>[5x]GVSKTFKDKCAS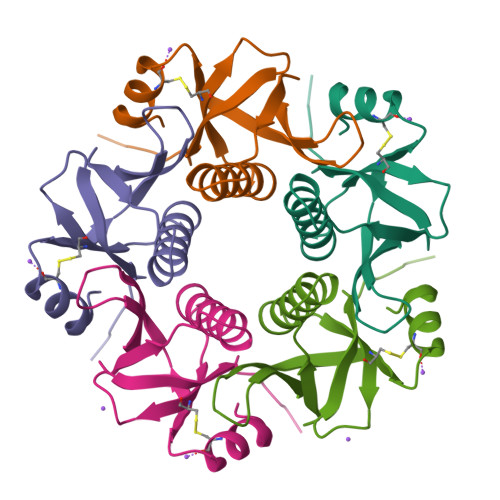TTAKLVQSVQLVNISSDVNKDSKGIYISSSAGKTWFIPGGQYYPDNYLSNEMRKIAMAAVLSNVRVNLCASEAYTPNHVWAIELAPHHHHHH>MVGAGAYAYKTMKEDEKRYNERISGLGLTPEQKQKKAALSASEGEEVPQDKAPSHVPFLLIGGGTAAFAAARSIRARDPGARVLIVSEDPELPYMRPPLSKELWFSDDPNVTKTLRFKQWNGKERSIYFQPPSFYVSAQDLPHIENGGVAVLTGKKVVQLDVRDNMVKLNDGSQITYEKCLIATGGTPRSLSAIDRAGAEVKSRTTLFRKIGDFRSLEKISREVKSITIIGGGFLGSELACALGRKARALGTEVIQLFPEKGNMGKILPEYLSNWTMEKVRREGVKVMPNAIVQSVGVSSGKLLIKLKDGRKVETDHIVAAVGLEPNVELAKTGGLEIDSDFGGFRVNAELQARSNIWVAGDAACFYDIKLGRRRVEHHDHAVVSGRLAGENMTGAAKPYWHQSMFWSDLGPDVGYEAIGLVDSSLPTVGVFAKATAQDNPKSATEQSGTGIRSESETESEASEITIPPSTPAVPQAPVQGEDYGKGVIFYLRDKVVVGIVLWNIFNRMPIARKIIKDGEQHEDLNEVAKLFNIHEDLEVLFQ[2x]

A 60-kDa FAD-dependent oxidoreductase, AIF allosterically switches between two distinct redox states. NADH binding by the oxidized AIF monomer reduces its FAD cofactor at a centralized active site, allosterically disrupting hydrogen bond networks to release a 50-residue surface loop (C-loop) and stimulate dimerization at the AIF surface. Oxidized NAD+ and reduced FADH– form a long-lived charge-transfer complex (CTC), which stabilizes and maintains the reduced dimeric state of AIF. NADH-activated AIF dimers support import of OXPHOS subunits by CHCHD4 and are critical for mitochondrial function.

To understand how SAXS CX1 and CX2 chemotypes engage AIF and enable dimerization, we crystallized select fragment hits with the W196A dimer-permissive mutant and wild-type AIF. Crystal structures of the W196A mutant bound to CX1 fragments and the underlying 4-aminoquinoline (4AQ) scaffold revealed that these scaffolds localize to the NADH active site, mirroring the native NADH ligand, as do CX1 and CX2 scaffolds bound to the wild-type protein. To accommodate this amine interaction, the aromatic side chain of F482 must rotate out of the binding site. Aligned with this, AIF structures with CX1 and CX2 ligands exhibiting partial occupancy indicate mixed orientations of the F482 aromatic ring. Crystallographic complexes of CX1 and CX2 fragments with AIF(W196A) (C12, D3 and D1) or wild-type AIF (C9, C11 and D7) reveal stabilizing active site contacts and sources of steric interference that correlate with AIF dimerization rates. By contrast, methyl substitution at position 3 (fragments C9 and C11) and methoxy substitution at position 6 (fragment D7) slow allosteric transition. Introducing methyl at position 3 for fluorinated analogs C9 and C11 prevents formation of a C12-like fluorine-π contact, as the methyl (C9) or amine (C11) of the rotated scaffold will clash with L311 on the opposite side of the active site. In their observed orientation, the methyl substitutions interfere with aromatic edge contacts to F482 and H454, which presumably slows stimulated AIF dimerization.> MTFEEKLSKIYNEIANEISSMIPVEWEKVYTMAYIDDGGGEVFFNYTKPGSDDLNYYTNIPKEYNISVQVFDDLWMDLYDLFEELRDLFKEEDLEPWTSCEFDFTREGELKVSFDYIDWINSEFGQIGRQNYYKYRKFGILPETEYEINKVKEIEQYIKELE;> PNYTKVEFGEHYARLRPKKLKANIEYTTPTGHIYRTDHKGRIKEVYVDNLSLKDGDRNSHAQRTVGGEDRLPDDDGGHLIARMFGGSKDIDNLVAQSKFINRPFKEKGHWYNLEKEWQEFLNSGKEVKNIKMEVKYSGNSQRPTIFKVEYEINGERNIRRILNK

Toxin EsaD secreted by some S. aureus strains through the type VII secretion system (T7SS) specifically kills those strains lacking the antitoxin EsaG. EsaD is a toxin secreted in a T7SS machinery-dependent manner by S. aureus. Here we report the structures of EsaG, the nuclease domain of EsaD and their complex, which together reveal an inhibition mechanism that relies on significant conformational change of the toxin. The major contribution of this study is the discovery of an inhibitory mechanism in the toxin-antitoxin module that is based on a significant structural deformation of the toxin, where the central β-sheet of the nuclease domain of EsaD is split by EsaG into two fragments.

The crystal structures were determined at resolutions of 2.30 Å for the nuclease domain of EsaD (residues 440–614) and 2.60 Å for the EsaG-EsaD (residues 450–614, hereafter referred as EsaDc) complex, respectively. However, the toxin, EsaD, undergoes significant conformational changes during the complex formation. The central 6-stranded β-sheet of EsaDc is split into two independent fragments: the N-terminal fragment (NF) consists of β1-3, which merges with the central β-sheet of EsaG through β4’ of EsaG and β3 of EsaDc; In the C-terminal fragment, αB from the ββα-metal finger and β6-8 interact with EsaG from the other side of the central β-sheet of EsaG. We could not trace the Mg2+ ion in the catalytic center, the long loop flanking the N-terminus of NF (Residues 450–468) and part of the ββα-metal finger motif, including αA to the finger loop (Residues 504–556). Noticeably, the N-terminus and C-terminus of the missing ββα-metal finger motif locate on two opposite sides of EsaG, with a linear distance of about 44 Å. These observations indicated that the separation of NF and CF of EsaDc by EsaG may stretch the originally folded ββα-metal finger motif to make it become a disordered loop and stride across such a long distance, thus abolishing the DNase activity of EsaDc. All the secondary structure elements of EsaDc are involved in the direct association with EsaG, mainly through hydrogen bonds, salt bridges and hydrophobic packing interactions. The CF binding is contributed collectively by αB and β6-8 of EsaDc, burying a solvent-accessible surface area of 3825 Å2, which is much larger than that of the 2461 Å2 in the NF binding site. Even though there is only one EsaDc-EsaG complex in the asymmetric unit, gel-filtration experiments showed that the complex was eluted at a volume corresponding to a molecular weight of 80 KD, close to that of two EsaDc-EsaG dimers. The results showed that strong signal of cross-linked product was generated only by EsaGQ69C in the presence of EsaDc, suggesting that two EsaDc-EsaG dimers form a tetramer through the CFs.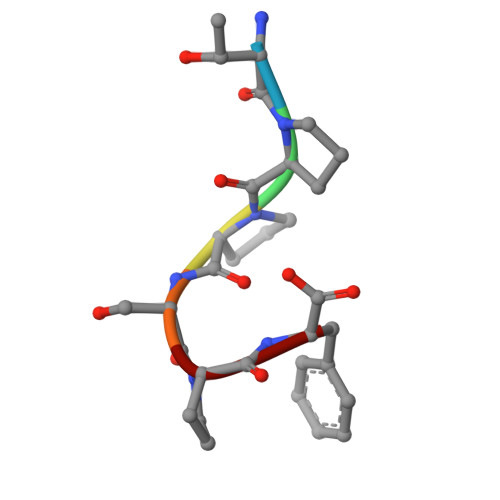> TPPSPF METHYL[CYCLO-7[(2R)-((N-VALYL)AMINO)-2-(HYDROXYL-(1S)-1-METHYLOXYCARBONYL-2-PHENYLETHOXY)PHOSPHINYLOXY-ETHYL]-1-NAPHTHALENEACETAMIDE] 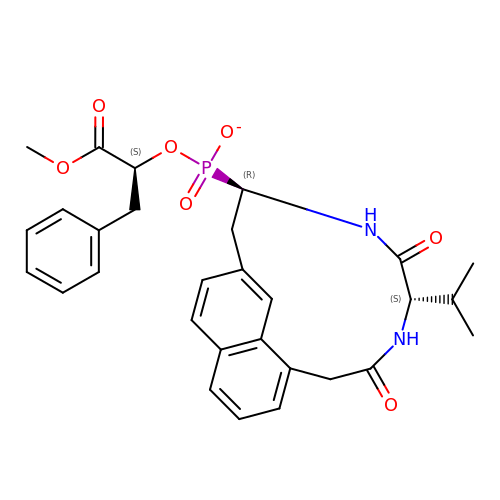| C29 H32 N2 O7 P | BJANYCOFDSBOJK-OIKPOIBNSA-M>MKVP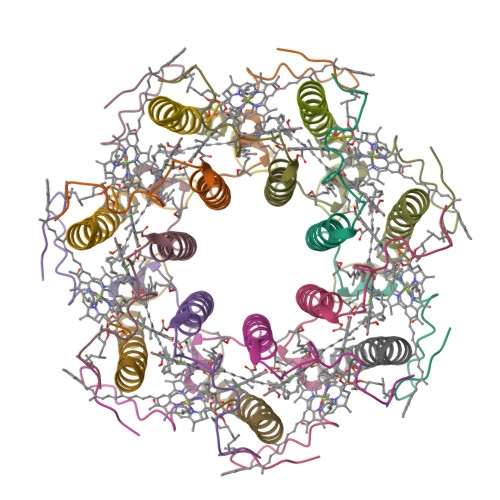VMMADESIATINHPEDDWKIWTVINPATWMVPFFGILFVQMWLIHSYALSLPGYGFKDSVRVAQPA[7x];>[7x]ADPKAANLSGLTDAQAKEFHEHWKHGVWSWVMIASAVHVVTWIYQPWF>MVKVDLESKRYGEKLKEVFLMLDNNVVECIKEITESSRNGKLVFFVGAGVSTLSDYPQWWRLVDKYHEELYGSPKKGNYSSDEYLRIPQIFYNVKGEMAFDGILKDFFQVDKPTNPIHDKILAMNPAHVITTNYDNLIDTACWKRGKYFSVISAEEDVANATSSRYLLKVAGDFRKGFKGENVVLKEDDYLNYDQNYPLISNLMKTIIATHTIVFIGYGLGDYNINMLLNWVRKLQKDSFHKPFFIRTDPSPIENETLIYYENKGLRIIDAASLIDSNEYDYLERYSAVMDLLIESQENKFITKDDEVIDYIYGKISPLFALQYIRKIDLKHVFEYDYHFEVNGTVVR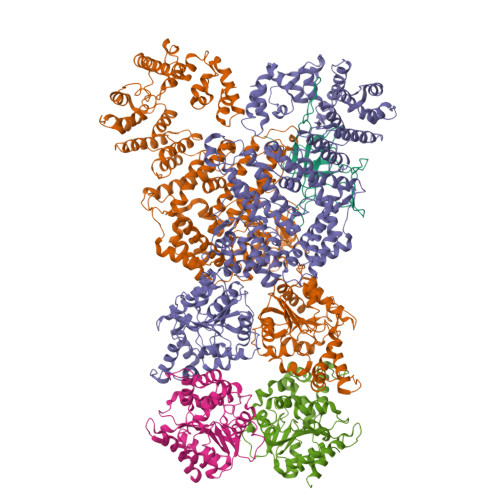HKNKGFGYMERFFELKESCDERSKLSKKQYERFNALFNFFEKNGVICMAKDAGTLNTSIEINSLAYHGKYDVMKKFIEEQSVSIEDDYKKAFFLACLGRWEESYDLYSNIILNSIDESNGCVYYLSQINRYRIYQSITQAVTQFNGLGLLTFGRHYKPFTDEFLARIEREMTNFNIDDLFNGMPFEFQKKYKILEFLSDNQFLYDDTVKLFELTNKVRSEMSEGSYSFGMSSDIVVLLRLYDNLRFLYENCLWSVSFHEFHQYIRNSMSLLIEKAEYERTRDIDELGFSFFGKKSGFFMEYYDFVNISRHFKIDDIKNLERSCSIDKIRFGEQEKIEEYLVGIAEEITKQFSANGMNVVFYTQFISEAKAALYFAKYVKLSEEGLGKIVKALLFYFPERDLDIGKRYVWLERLTKCNELPKSIISIIDDFLVLQAEKHIDQNYSEVSSNGLYSRDYGALIKHFEKNFISKRLSEITLCLTQDKQKQIDFLFKLLPLLSTNAKSHLLSFKSVENINDLMNGIRIGLIDEFTPEHEELIIEYLETRKVNYIVEKEKGIQTFSSNDYMSTFGIWYFLEEINNSKMEEFIGMDDQYDFFVDPENFDYKKFIPSWLKNYNDKLLGKIAGNKHMKHHVIEVLKERVKNSNDKRYLEILMNYFI[4x];> MKTVIQDTADVYFKRKSDGKLVFTAEAQTASFSQAISEEKLRGGIGNKPLYILKSEKEINLTVKNAFFDLEWLAMTQGETIQEETKVKVFDREHGLIVDDTNKVTLKGKPVSDVTFYNKKGLTYKIAVSTDGTYTIPTAFAAAKDKLTAVYQIEKVGRRLAIKASKFSERYEVEYRTIAYNPDTEEVYSDIYIQFPNVSPSGEFEMSLENGNALAPEIKFEALADTDTDEMAVVIEASRDENTAAPVEDTTGSTQSSDLGGTTE(3S,5R,6S,7R,8R,11R,12S,13R,14S,15S)-6-HYDROXY-5,7,8,11,13,15-HEXAMETHYL-4,10-DIOXO-14-{[3,4,6-TRIDEOXY-3-(DIMETHYLAMINO)-BETA-D-XYLO-HEXOPYRANOSYL]OXY}-1,9-DIOXASPIRO[2.13]HEXADEC-12-YL 2,6-DIDEOXY-3-O-METHYL-ALPHA-L-ARABINO-HEXOPYRANOSIDE | C35 H61 N O12 | 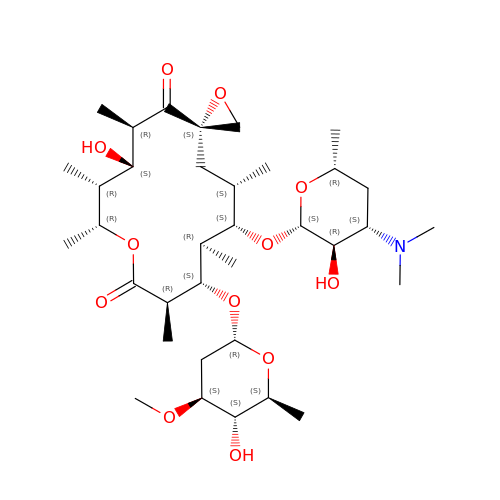RZPAKFUAFGMUPI-KGIGTXTPSA-N>GSKVEDPKDFPSELLSFLSHAVFSNRTLACFAIYTTKEKAALLYKKIMEK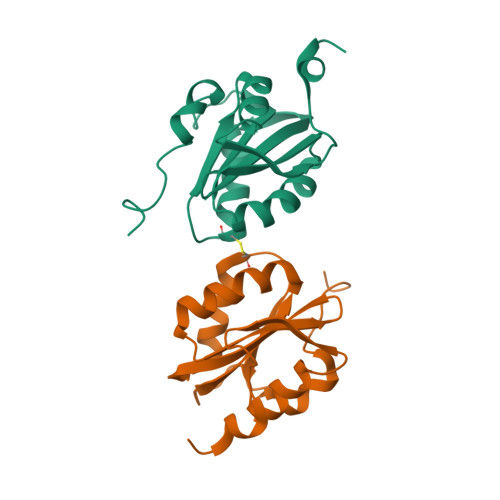YSVTFISRHNSYNHNILFFLTPHRHRVSAINNYAQKLCTFSFLICKGVNKEYLMYSALTRDPFSVIEESLPGGLKEHDFNPESS[2x]>MPMFIVNTNVPRASVPDGFLSELTQQLAQA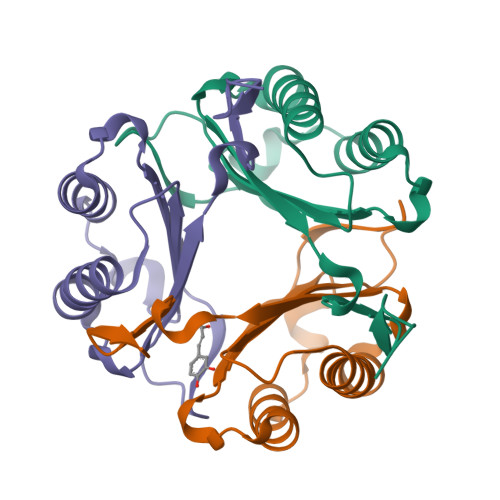TGKPPQYIAVHVVPDQLMAFGGSSEPCALCSLHSIGKIGGAQNRSYSKLLCGLLAERLRISPDRVYINYYDMNAANVGWNNSTFALEHHHHHH[3x]>ADTIVAVELDTYPNTDIGDPSYPHIGIDIKSVRSKKTAKWNMQNGKVGTAHIIYNSVDKRLSAVVSYPNADSATVSYDVDLDNVLPEWVRVGLSASTGLYKETNTILSWSFTSKLKSNSTHETNALHFMFNQFSKDQKDLILQGDATTGTDGNLELTRVSSNGSPQGSSVGRALFYAPVHIWESSAVVASFEATFTFLIKSPDSHPADGIAFFISNIDSSIPSGSTGRLLGLFPDAN[4x];>GWYN[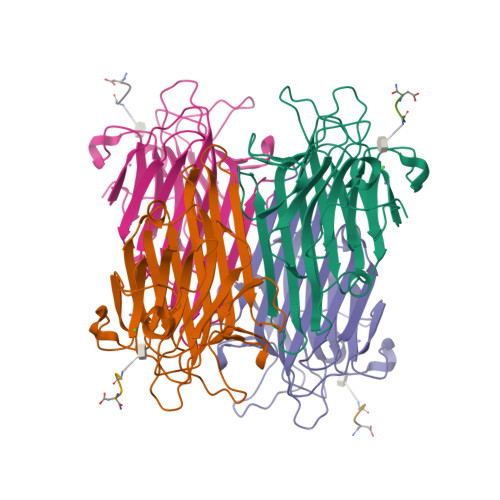4x]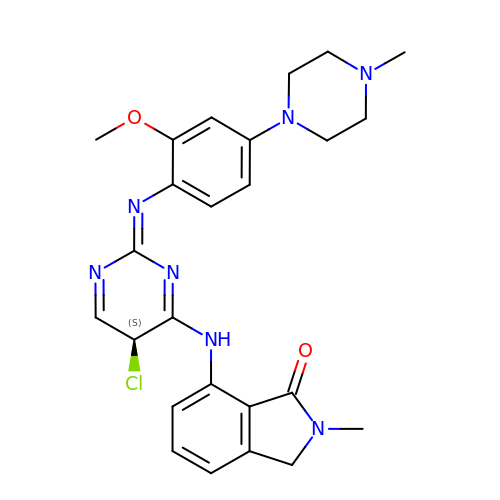7-{[(2Z,5S)-5-CHLORO-2-{[2-METHOXY-4-(4-METHYLPIPERAZIN-1-YL)PHENYL]IMINO}-2,5-DIHYDROPYRIMIDIN-4-YL]AMINO}-2-METHYL-2,3-DIHYDRO-1H-ISOINDOL-1-ONE | C25 H28 Cl N7 O2 | YKRBTLCKGPASPO-SFHVURJKSA-N> GAMESKKRQWALEDFEIGRPLG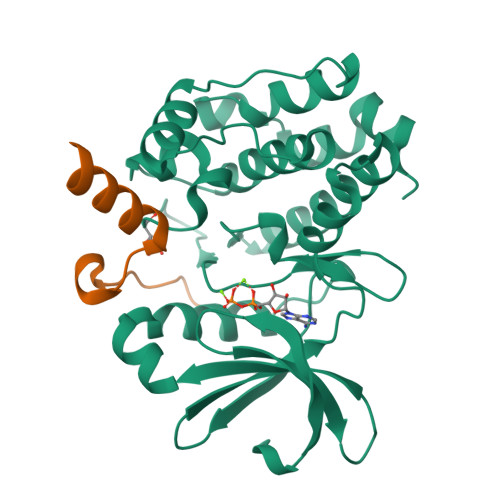KGKFGNVYLAREKQSKFILALKVLFKAQLEKAGVEHQLRREVEIQSHLRHPNILRLYGYFHDATRVYLILEYAPLGTVYRELQKLSKFDEQRTATYITELANALSYCHSKRVIHRDIKPENLLLGSAGELKIADFGWSVHAPSSRRTTLAGTLDYLPPEMIEGRMHDEKVDLWSLGVLCYEFLVGKPPFEANTYQETYKRISRVEFTFPDFVTEGARDLISRLLKHNPSQRPMLREVLEHPWITANSSKPSNAQNKESASKQS;> SFYPDEDDFYFGGPDSTPPGEDIWKKFELLPTPPLSPSRGFAEHSSEPPSWVTEMLLENELWG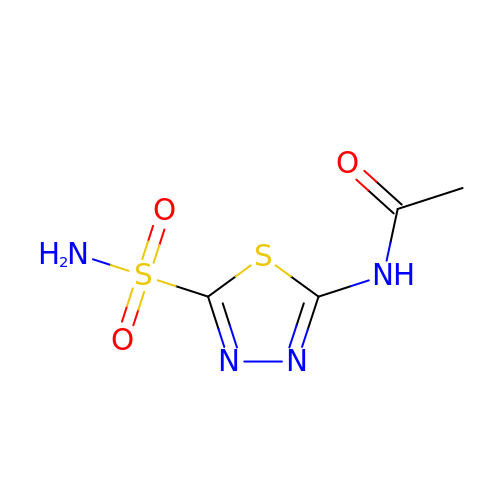5-ACETAMIDO-1,3,4-THIADIAZOLE-2-SULFONAMIDE | C4 H6 N4 O3 S2 | BZKPWHYZMXOIDC-UHFFFAOYSA-N> MAYTRSKIVDLVDGKIDPDTLHQMLSTPKDPERFVTYVEILQERMPWDDKIILPLGPKLFIVQQKVSKKWTVRCECGHDFCDWKDNWKLSARVHVRDTPQ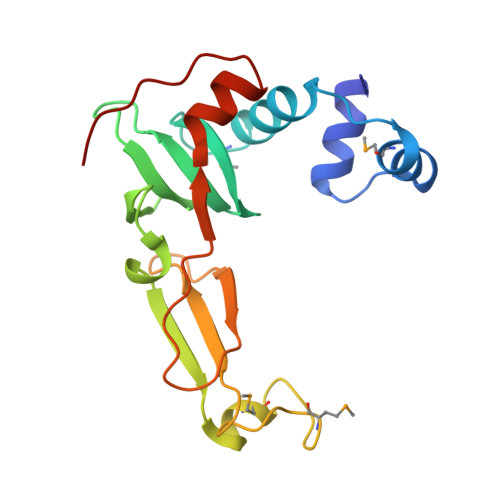KMEEIYPRLMAPTPSWQVIREYFCPECGTLHDVEAPTPWYPVIHDFSPDIEGFYQEWLGLPVPERADA>MVSLEKNDHLMLARQLPLKSVALILAGGRGTRLKDLTNKRAKPAVHFGGKFRIIDFALSNCINSGIRRMGVITQYQSHTLVQHIQRGWSFFNEEMNEFVDLLPAQQRMKGENWYRGTADAVTQNLDIIRAYKAEYVVILAGDHIYKQDYSRMLIDHVEKGARCTVACMPVPIEEASAFGVMAVDENDKIIEFVEKPANPPSMPNDPSKSLASMGIYVFDADYLYELLEEDDRDENSSHDFGKDLIPKITEAGLAYAHPFPLSCVQSDPDAEPYWRDVGTLEAYWKANLDLASVVPELDMYDRNWPI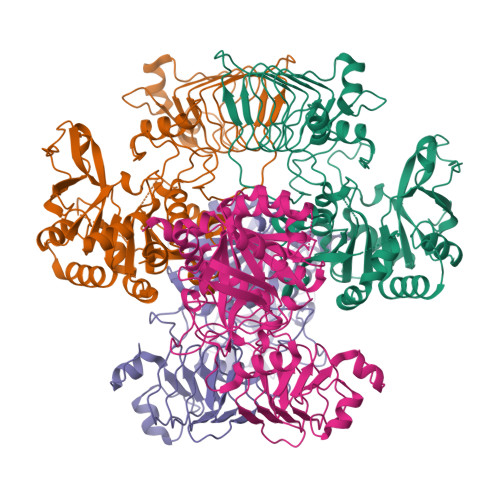RTYNESLPPAKFVQDRSGSHGMTLNSLVSGGCVISGSVVVQSVLFSRVRVNSFCNIDSAVLLPEVWVGRSCRLRRCVIDRACVIPEGMVIGENAEEDARRFYRSEEGIVLVTREMLRKLGHKQER[8x]> QPKTFTVRIVTMDAEMEFNCEMKWKGKDLFDLVCRTLGLRETWFFGLQYTIKDTVAWLKMDKKVLDHDVSKEEPVTFHFLAKFYPENAEEELVQEITQHLFFLQVKKQILDEKVYCPPEASVLLASYAVQAKYGDYDPSVHKR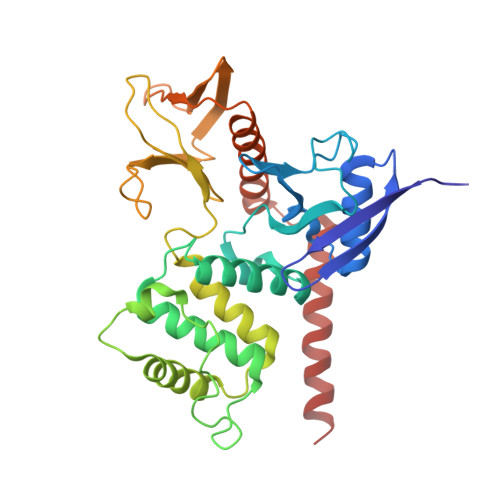GFLAQEELLPKRVINLYQMTPEMWEERITAWYAEHRGRARDEAEMEYLKIAQDLEMYGVNYFTIRNKKGTELLLGVDALGLHIYDPENRLTPKISFPWNEIRNISYSDKEFTIKPLDKKIDVFKFNSSKLRVNKLILQLCIGNHDLFMRRRKADSLEVQQMKAQAREEKARKQMERQRLA> MINMODELKKLFLVFWWHMHQPLYREPYTGEYLLPWTFFHAVKDYYDMPAYLKDFEIKLNFNLTPVLIDQIQEYAQGKAKDVFLEAIRKDPDDLEKEEVEKLIEFTKLNYEKPIYRFERIRELMNKEKLNREELLDLQTLNLLAWCGRTLRKDLKDLLNKGRNYTQEEKEYVLNKYFEIIKKTLSIYREIKEEGKGSVSTSPYYHPLIPILLNPNCVYETTPNVKIPDFAVSFREDASKHVELAKEKYFEIFGEHPVYMWPPEASVSNEALELYYEKGINMLATDEVILKNSVERASPYLRYYFRELISVFFRD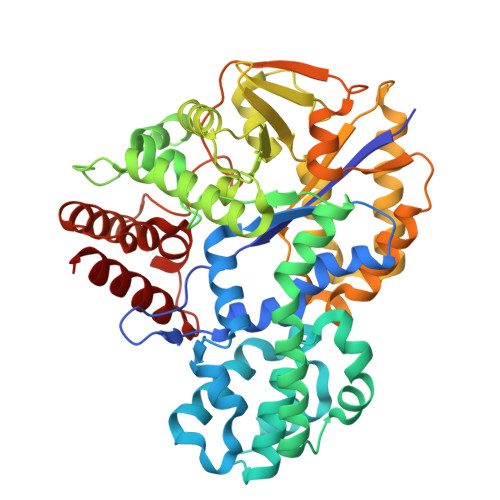KTLSDLIGFSYHAWNAEDAVRDFIGRLKKIHESVDFQPVVFVVLDGENCWEYYEENGIPFLEKLYSTLEKEEWIETLTLEEAMRKEDVKTEVIESVKAGTWFDGNFLKWIGNKEKNEYWKILIEAKKKAKNDYILVAEGSDWFWWQGEEKAPFVEVFDKLFRSFVRRAQE> GPY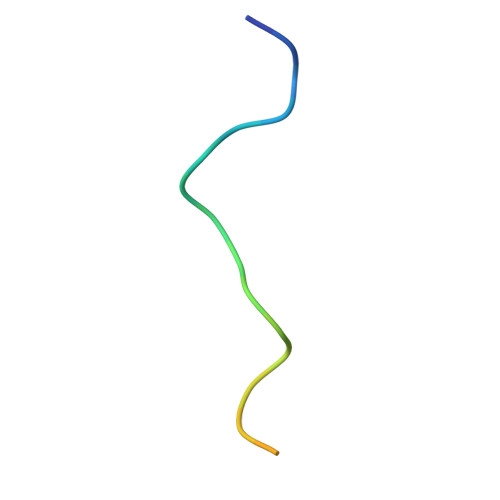AGPLERQRPLKVRAKLPRQE> SSQSISPMRSISENSLVAMDFSGQKSRVIENPTEALSVAVE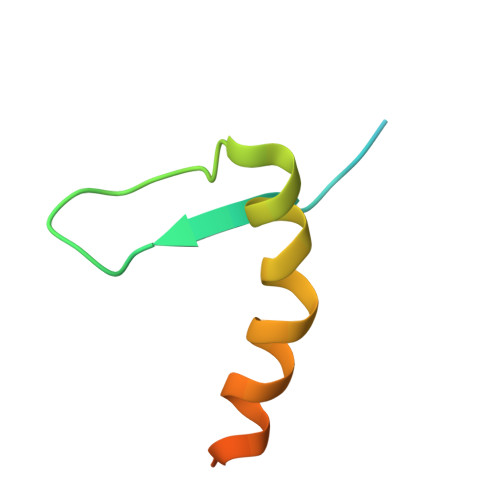EGLAWRKKGSLRLGTHGS1,1'-benzene-1,4-diylbis(1H-pyrrole-2,5-dione) | C14 H8 N2 O4 | 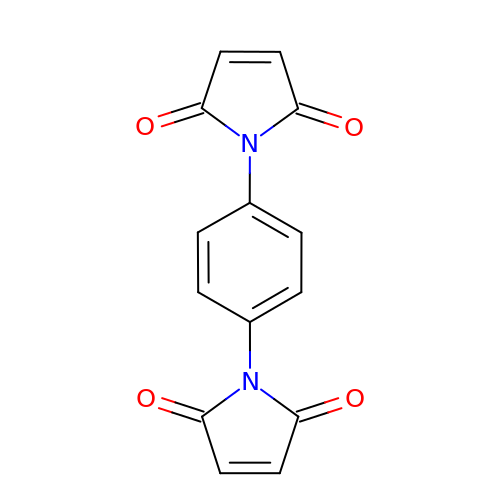AQGZJQNZNONGKY-UHFFFAOYSA-N>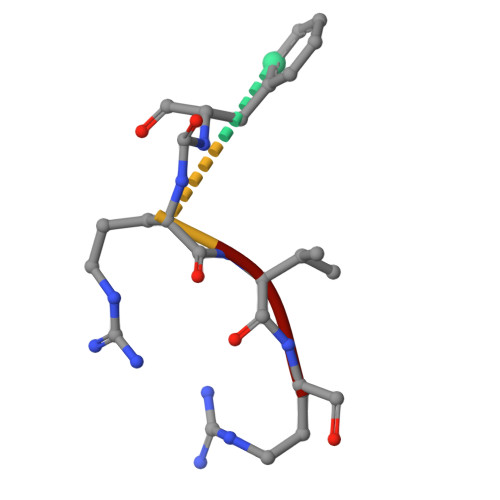 FRVR>[2x]MSDKLPYKVADIGLAAWGRKALDIAENEMPGLMRMREMYSASKPLKGARIAGCLHMTVETAVLIETLVALGAEVRWSSCNIFSTQDHAAAAI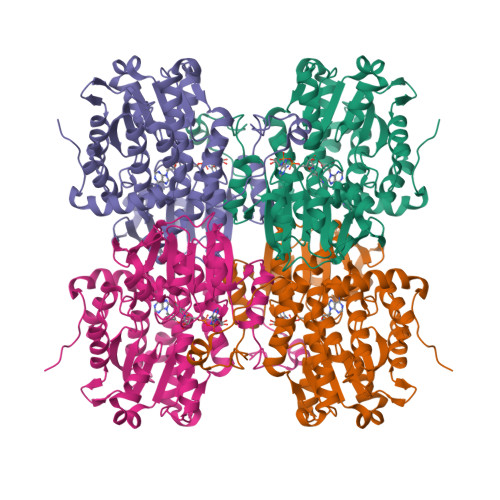AKAGIPVFAWKGETDEEYLWCIEQTLHFKDGPLNMILDDGGDLTNLIHTKYPQLLSGIRGISEETTTGVHNLYKMMSNGILKVPAINVNDSVTKSKFDNLYGCRESLIDGIKRATDVMIAGKVAVVAGYGDVGKGCAQALRGFGARVIITEIDPINALQAAMEGYEVTTMDEACKEGNIFVTTTGCVDIILGRHFEQMKDDAIVCNIGHFDVEIDVKWLNENAVEKVNIKPQVDRYWLKNGRRIILLAEGRLVNLGCAMGHPSFVMSNSFTNQVMAQIELWTHPDKYPVGVHFLPKKLDEAVAEAHLGKLNVKLTKLTEKQAQYLGMPINGPFKPDHYRY> GSHMAEHDAAAEGLGQLTLTMCLSGSVSSVAGPHMAAWLSSAGVGRLHVALTPSAQQFVTTNSLRPFVNGSVLTDETVWSAGGAPHVRI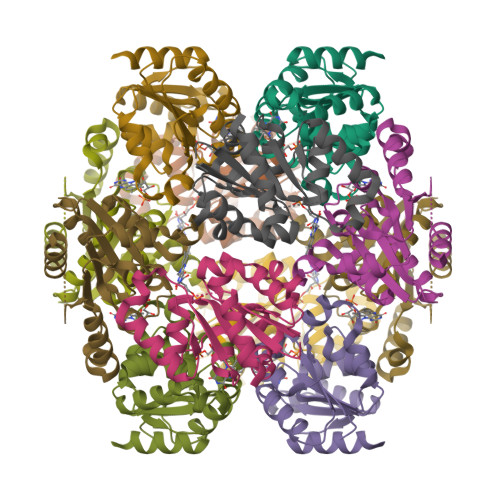AAESDAVVVAPATAATLGKLANGICDNIVTQIVMAAECPVILAPVMNPAMLAKPAVRRNLDALRAEGFVVAEPGQGVNATNGRWEAGSMADFRSVFAVALKSAAERKSASD>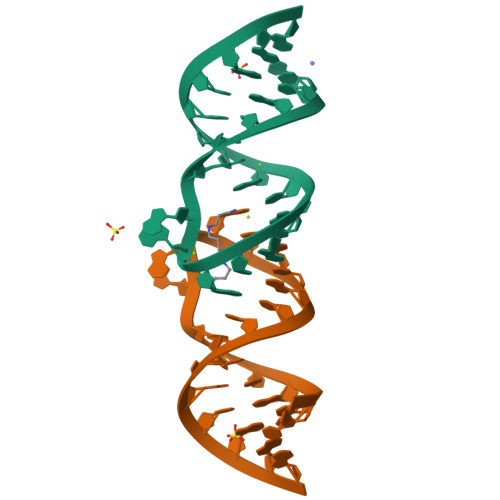[2x]CUUGCUGAGGUGCACACAGCAAG> MSRPLSDQEKRKQISVRGLAGVENVTELKKNFNRHLHFTLVKDRNVATPRDYYFALAHTVRDHLVGRWIRTQQHYYEKDPKRIYYLSLEFYMGRTLQNTMVNLALENACDEATYQLGLDMEELEEIEEDAGLGNGGLGRLAACFLDSMATLGLAAYGYGIRYEFGIFNQKICGGWQMEEADDWLRYGNPWEKARPEFTLPVHFYGRVEHTSQGAKWVDTQVVLAMPYDTPVPGYRNNVVNTMRLWSAKAPNDFNLKDFNVGGYIQAVLDRNLAENISRVLYPNDNFFEGKELRLKQEYFVVAATLQDIIRRFKSSKFGCRDPVRTNFDAFPDKVAIQLNDTHPSLAIPELMRVLVDLERLDWDKAWEVTVKTCAYTNHTVLPEALERWPVHLLETLLPRHLQIIYEINQRFLNRVAAAFPGDVDRLRRMSLVEEGAVKRINMAHLCIAGSHAVNGVARIHSEILKKTIFKDFYELEPHKFQNKTNGITPRRWLV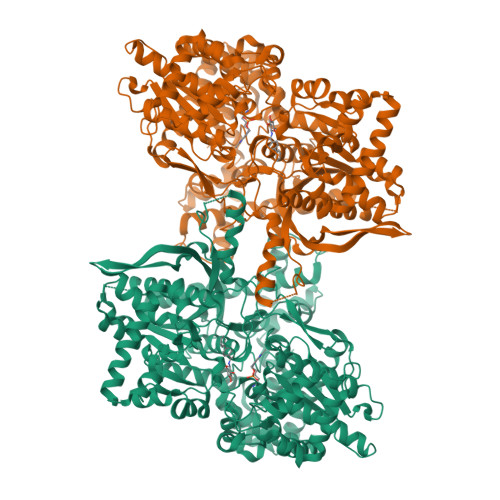LCNPGLAEIIAERIGEEYISDLDQLRKLLSYVDDEAFIRDVAKVKQENKLKFAAYLEREYKVHINPNSLFDVQVKRIHEYKRQLLNCLHVITLYNRIKKEPNKFVVPRTVMIGGKAAPGYHMAKMIIKLITAIGDVVNHDPVVGDRLRVIFLENYRVSLAEKVIPAADLSEQISTAGTEASGTGNMKFMLNGALTIGTMDGANVEMAEEAGEENFFIFGMRVEDVDRLDQRGYNAQEYYDRIPELRQIIEQLSSGFFSPKQPDLFKDIVNMLMHHDRFKVFADYEEYVKCQERVSALYKNPREWTRMVIRNIATSGKFSSDRTIAQYAREIWGVEPSRQRLPAPDEKIP>GPAFEFAVAMMKRNSSTVKTEYGEFTMLGIYDRWAVLPRHAKPGPTILMNDQEVGVLDAKELVDKDGTNLELTLLKLNRNEKFRDIRGFLAKEEVEVNEAVLAINTSKFPNMYIPVGQVTEYGFLNLGGTPTK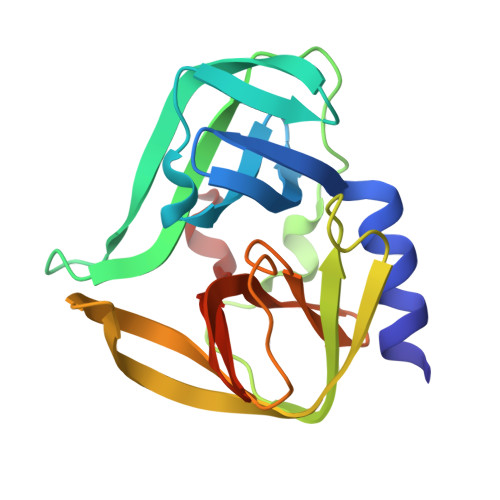RMLMYNFPTRAGQCGGVLMSTGKVLGIHVGGNGHQGFSAALLKHYFNDEQ[2x]>[3x]AMPLDAGGQNSTQMVLAPGASIFRCRQCGQTISRRDWLLPMGG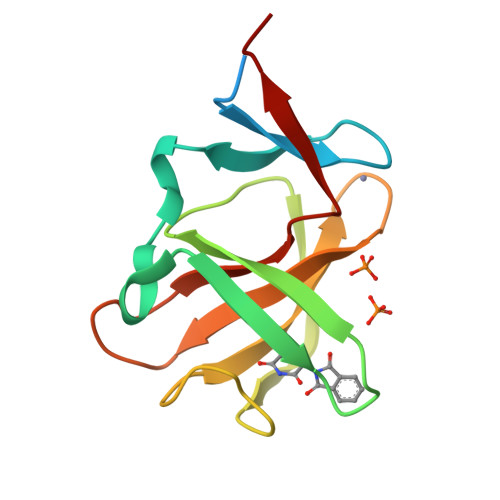DHEHVVFNPAGMIFRVWCFSLAQGLRLIGAPSGEFSWFKGYDWTIALCGQCGSHLGWHYEGGSQPQTFFGLIKDRLAEGPAD>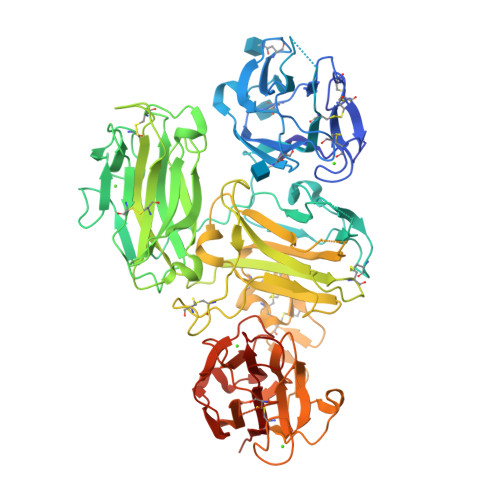 EIHSDSVILRDDFDSYQQLELNPNIWVECSNCEMGEQCGTIMHGNAVTFCEPYGPRELTTTCLNTTTASVLQFSIGSGSCRFSYSDPSITVSYAKNNTADWIQLEKIRAPSNVSTVIHILYLPEEAKGESVQFQWKQDSLRVGEVYEACWALDNILVINSAHREVVLEDNLDPVDTGNWLFFPGATVKHSCQSDGNSIYFHGNEGSEFNFATTRDVDLSTEDIQEQWSEEFESQPTGWDILGAVVGADCGTVESGLSLVFLKDGERKLCTPYMDTTGYGNLRFYFVMGGICDPGVSHENDIILYAKIEGRKEHIALDTLTYSSYKVPSLVSVVINPELQTPATKFCLRQKSHQGYNRNVWAVDFFHVLPVLPSTMSHMIQFSINLGCGTHQPGNSVSLEFSTNHGRSWSLLHTECLPEICAGPHLPHSTVYSSENYSGWNRITIPLPNAALTRDTRIRWRQTGPILGNMWAIDNVYIGPSCLKFCSGRGQCTRHGCKCDPGFSGPACEMASQTFPMFISESFGSARLSSYHNFYSIRGAEVSFGCGVLASGKALVFNKDGRRQLITSFLDSSQSRFLQFTLRLGSKSVLSTCRAPDQPGEGVLLHYSYDNGITWKLLEHYSYVNYHEPRIISVELPDDARQFGIQFRWWQPYHSSQGEDVWAIDEIVMTSRLENLYF>[2x]MTRETERFPAREFQRDLLDWFARERRDLPWRKDRDPYKVWVSEVMLQQTRVETVIPYFEQFIDRFPTLEALADADEDEVLKAWEGLGYYSRVRNLHAAVKEVKTRYGGKVPDDPDEFSRLKGVGPYTVGAVLSLAYGVPEPAVDGSVMRVLSRLFLVTDDIAKPSTRKRFEQIVREIMAYENPGAFNEALIELGALVCTPRRPSCLLCPVQA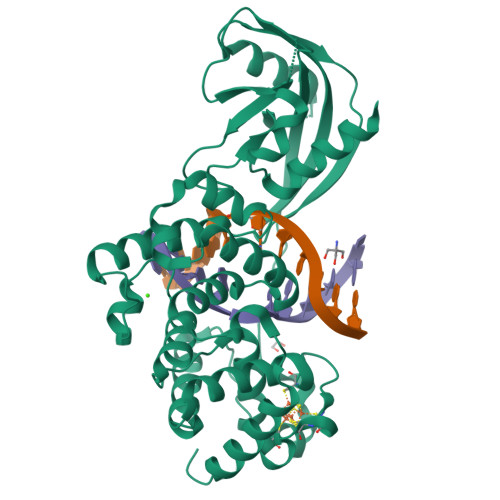YCQAFAEGVAEELPVKMKKTAVKQVPLAVAVLADDEGRVLIRKRDSTGLLANLWEFPSCETDGADGKEKLEQMVGEQYGLQVELTEPIVSFEHAFSHLVWQLTVFPGRLVHGGPVEEPYRLAPEDELKAYAFPVSHQRVWREYKEWASGVRRP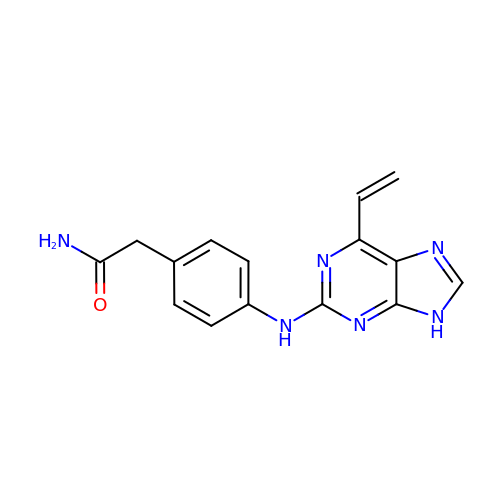2-[4-[(6-ethenyl-9~{H}-purin-2-yl)amino]phenyl]ethanamide | C15 H14 N6 O | LSWHKQJKPIFFMY-UHFFFAOYSA-N> MITHRPRGIEHPYARSLDQLYPAIPIAGQSLTIGATTSGPCSRMRCFVLWPEHEQVFDMSPVNGTDSDAALLAGGEGHLAAAQQAALDADNGWQTSIPHLPDQDATYYFEALTLDGRTETSESFPLTPSHWSAEPVGHIDIDGDRFIPDSPLWLVSSAGTHRVKFALRIEGDEHVVGFGERYDQLDQRGLRLDSVVFEQYKAQGKH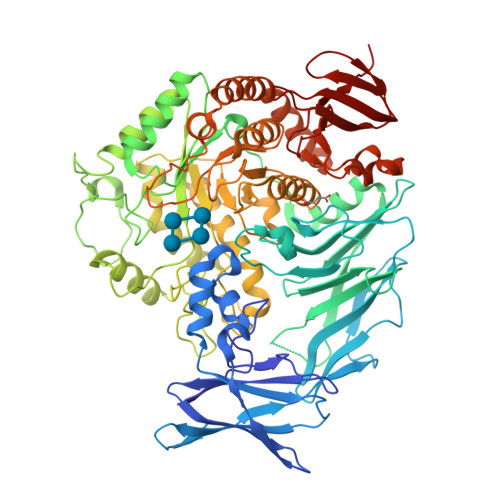HRTYLPMPFAQVVNEAGRAWGFHVETTRRTWYDVAATVSDRILIEVDLGFEAEKTPVVRVNTWSGSPTDVLNGFLDVAGRPAEMPEWIFGLWASGNEWNTQSLVMEQMDRHRNEGIPVSVVVIEAWSDEEGFTIFRDARYVPNQGQPHRGPDFTYPSDGAWPDPAGMIRELHERGIRVILWQIPLQKTDDDLGPEALAQGNALIASGHVVKEPDGTPYKNRGWWFPNALMPDLSTEAGRQWWTEQRRYLVEDLDIDGFKTDGGEHAWGSDLRYEDGRRGDEGNNLYPVNYARAYGDLLRSAGKYPVTFSRSGFTGSQAHGLYWAGAEDSTWEAFRSSITAGITAGACGILYWGWDLAGFSGPVPEAELYARAFAAATFMPIMQYHSEFHHHELPLRDRTPWNVAEQTGCGELIDLARHYTRVREALRPYLVAQTRQCLQTGKPLMRAMFYDHADDPEIWAHPRQYMLGDELLINPVTAPGATTWTTYLPEGQWEDYWSGEVSEGGHLVTRAVGWDIIPVYRRVGAAL>[8x]SGSGMYRNFLKRVIDILGALFLLILTSPIIIATAIFIYFKVSRDVIFTQARPGLNEKIFKIYKFKTMSDERDANGELLPDDQRLGKFGKLIRSLSLDELPQLFNVLKGDMSFIGPRPLLVEYLPIYNETQKHRHDVRPGITGLAQVNGRNAISWEKKFEYDVYYAKNLSFMLDVKIALQTIEKVLKRSGVSKEGQATTEKFNGKN

pmcPhosphoglycosyl transferases (PGTs) catalyze the transfer of a phosphosugar group from a UDP-sugar substrate to a membrane-resident polyprenol phosphate (most commonly in bacteria undecaprenol or decaprenol phosphate) acceptor. PglC is a monotopic phosphoglycosyl transferase that embodies the functional core structure of the entire enzyme superfamily and catalyzes the first membrane-committed step in a glycoprotein assembly pathway. Catalysis proceeds via a covalent intermediate with both soluble and amphiphilic substrates remaining in aqueous and membrane environments, respectively.

In the current study, further insight is derived from the structure of selenomethionine (SeMet)-derivatized PglC co-crystallized with UDP. UDP was utilized in co-crystallization, as it significantly stabilized this PGT as shown by nanoscale differential scanning fluorimetry (nanoDSF). In contrast to I57M/Q175M PglC, the SeMet PglC has an asymmetric unit (ASU) comprising eight monomers rather than two per unit cell, allowing independent refinement. Although the resolution was low (3.01 Å), and the ligand was not stoichiometrically bound (10–20% occupancy of any ligand to the active site), it was possible to make correlations between the presence or absence of electron density and the loop conformations. When the eight copies of PglC in the ASU were overlaid, the mobile loop is the main region of structural divergence between the chains. In monomers G and H, which are closed, as well as A and B (intermediate conformation), a comparatively large number of electrons is present in the site where the nucleotide would be expected to bind. In contrast, monomers C, D, E, and F, which are open, all have significantly fewer electrons present. Analysis of the mobile loop in the context of active-site ligand occupancy shows that chains with a greater positive electron density were in a more closed conformation than those with little or no density. Monomers occupying the same position within each of the four lattice dimers do not always occupy the same mobile loop position; thus, the difference in the observed loop conformation is likely due to differential binding at the active site.>GPHMRVRLKAHYGGDILITSVDPTTTFQDLCEEVRDMCGLHQQHPLTLKWVDSEGDPCTVSSQMELEEAFRLACQGRDEVLIIHVFPSIPE[12x];>[12x]GPHMSLTVKAYLLGKEDAAREIRRFSFCCSPEPEAEAEAAAGPGPCERLLSRVAALFPALRPGG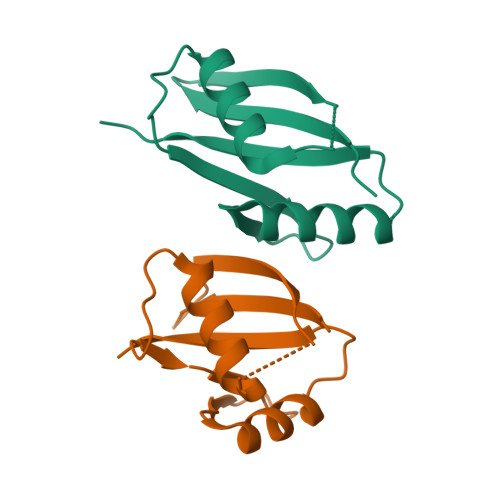FQAHYRAERGDLVAFSSDEELTMAMSYVKDDIFRIYIKEK> AADLADRFAELERRYDARLGVYVPATGTTAAIEYRADERFAFCSTFAAPLVAAVLHQNPLTHLDKLITYTSDDIRSISPVAQQHVQTGMTIGQLCDAAIRYSDGTAANLLLADLGGPGGGTAAFTGYLRSLGDTVSRLDAEEPELNRDPPGDERDTTTPHAIALVLQQLVLGNALPPDKRALLTDWMARNTTGAKRIRA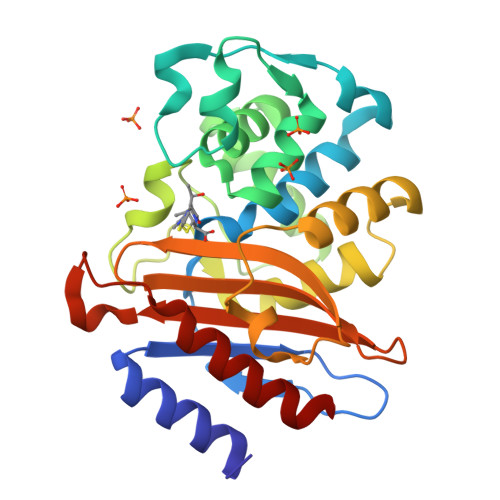GFPADWKVIDKTGTGDYGRANDIAVVWSPTGVPYVVAVMSDRAGGGYDAEPREALLAEAATCVAGVLA> MREFGNPLGDRPPLDELARTDLLLDALAEREEVDFADPRDDAL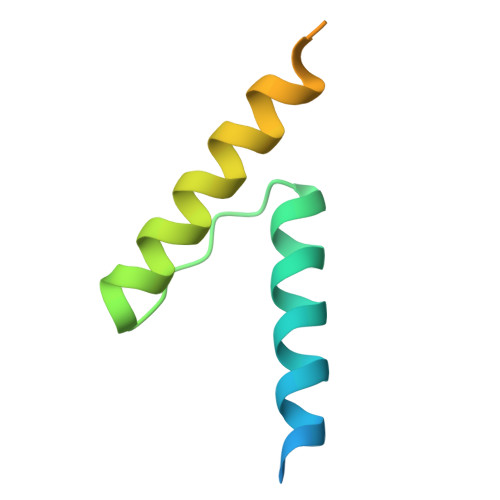AALLGQWRDDLRWPPASALVSQDEAVAALRAGVAQRR> MSGELSNRFQGGKAFGLLKARQERRLAEINREFLCDQKYSDEENLPEKLTAFKEKYMEFDLNNEGEIDLMSLKRMMEKLGVPKTHLEMKKMISE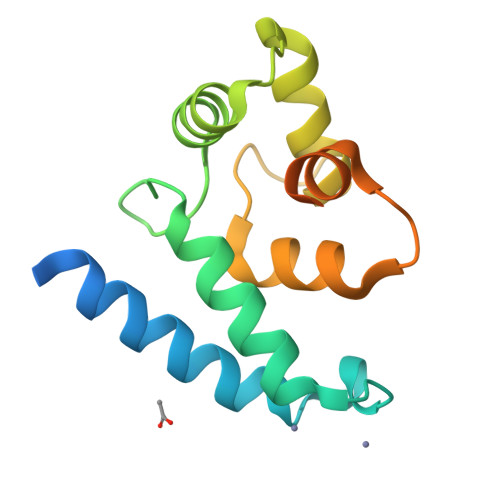VTGGVSDTISYRDFVNMMLGKRSAVLKLVMMFEGKANESSPKPVGPPPERDIASLP>[2x]MWSHPAVRKSSSKTIRSRSIWDDAHAMLEKAKAEGISTVWDRAAEQTPACKFCELGTTCRNCIMGPCRIANRKDGKMRLGVCGADADVIVARNFGRFIAGGAAGHSDHGRDLIETLEAVAEGKAPGYTIRDVAKLRRIAAELGVADAATRPAHDVAADLVTICYNDFGSRRNALAFLARAPQVRRDLWQRL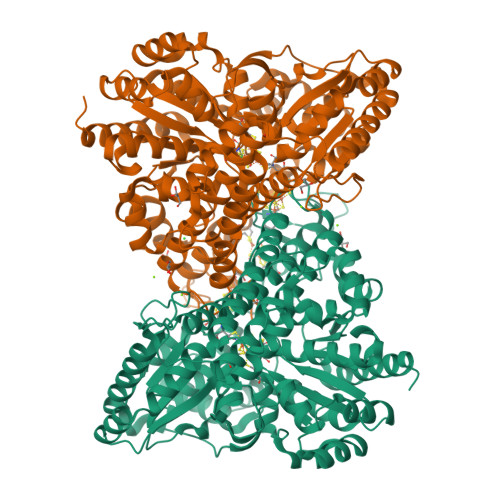GMTPRGVDREIAEMMHRTHMGCDNDHTSLLVHAARTALADGWGGSMIGTELSDILFGTPRPRQSTVNLGVLRKDAVNILVHGHNPVVSEMILAATREPAVRQAAQDAGAADINVAGLCCTGNELLMRQGIPMAGNHLMTELAIVTGAADAIVADYQCIMPSLVQIAACYHTRFVTTSPKGRFTGATHVEVHPHNAQERCREIVMLAIDAYTRRDPARVDIPSQPVSIMSGFSNEAILEALGGTPKPLIDAVVAGQIRGFVGIVGCNNPKIRQDSANVTLTRELIRRDIMVLATGCVTTAAGKAGLLVPEAASKAGEGLAAVCRSLGVPPVLHMGSCVDNSRILQLCALLATTLGVDISDLPVGASSPEWYSEKAAAIAMYAVASGIPTHLGLPPNILGSENVTAMALHGLQDVVGAAFMVEPDPVKAADMLEAHIVARRARLGLTS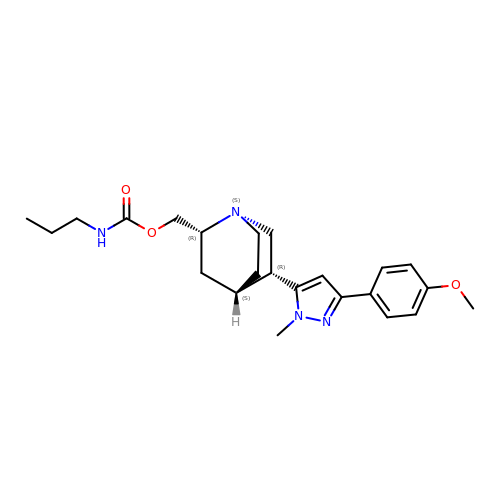[(1~{S},2~{R},4~{S},5~{R})-5-[5-(4-methoxyphenyl)-2-methyl-pyrazol-3-yl]-1-azabicyclo[2.2.2]octan-2-yl]methyl ~{N}-propylcarbamate | C23 H32 N4 O3 | WHTNZQHPDMCEMQ-NSHGMRRFSA-N> ALYTLITPAVLRTDTEEQILVEAHGDSTPKQLDIFVHDFPRKQKTLFQTRVDMNPAGGMLVTPTIEIPAKEVSTDSRQNQYVVVQVTGPQVRLEKVVLLSYQSSFLFIQTDKGIYTPGSPVLYRVFSMDHNTSKMNKTVIVEFQTPEGILVSSNSVDLNFFWPYNLPDLVSLGTWRIVAKYEHSPENYTAYFDVRKYVLPSFEVRLQPSEKFFYIDGNENFHVSITARYLYGEEVEGVAFVLFGVKIDDAKKSIPDSLTRIPIIDGDGKATLKRDTFRSRFPNLNELVGHTLYASVTVMTESGSDMVVTEQSGIHIVASPYQIHFTKTPKYFKPGMPYELTVYVTNPDGSPAAHVPVVSEAFHSMGTTLSDGTAKLILNIPLNAQSLPITVRTNHGDLPRERQATKSMTAIAYQTQGGSGNYLHVAITSTEIKPGDNLPVNFNVKGNANSLKQIKYFTYLILNKGKIFKVGRQPRRDGQNLVTMNLHITPDLIPSFRFVAYYQVGNNEIVADSVWVDVKDTCMGTLVVKGDNLIQMPGAAMKIKLEGDPGARVGLVAVDKAVYVLNDKYKISQAKI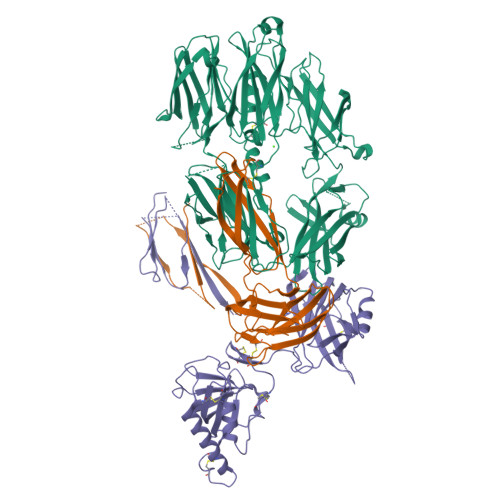WDTIEKSDFGCTAGSGQNNLGVFEDAGLALTTSTNLNTKQRSAAKCPQPAN;> EIQMPTHKDLNLDITIELPDREVPIRYRINYENALLARTVETKLNQDITVTASGDGKATMTILTFYNAQLQEKANVCNKFHLNVSVENIHLNAMGAKGALMLKICTRYLGEVDSTMTIIDISMLTGFLPDAEDLTRLSKGVDRYISRYEVDNNMAQKVAVIIYLNKVSHSEDECLHFKILKHFEVGFIQPGSVKVYSYYNLDEKCTKFYHPDKGTGLLNKICIGNVCRCAGETCSSLNHQERIDVPLQIEKACETNVDYVYKTKLLRIEEQDGNDIYVMDVLEVIKQGTDENPRAKTHQYISQRKCQEALNLKVNDDYLIWGSRSDLLPTKDKISYIITKNTWIERWPHEDECQEEEFQKLCDDFAQFSYTLTEFGCPT;> DDNEDGFIADSDIISRSDFPKSWLWLTKDLTEEPNSQGISSKTMSFYLRDSITTWVVLAVSFTPTKGICVAEPYEIRVMKVFFIDLQMPYSVVKNEQVEIRAILHNYVNEDIYVRVELLYNPAFCSASTKGQRYRQQFPIKALSSRAVPFVIVPLEQGLHDVEIKASVQEALWSDGVRKKLKVVPEGVQKSIVTIVKLDPRAKGVGGTQLEVIKARKLDDRVPDTEIETKIIIQGDPVAQIIENSIDGSKLN> MYDFTNC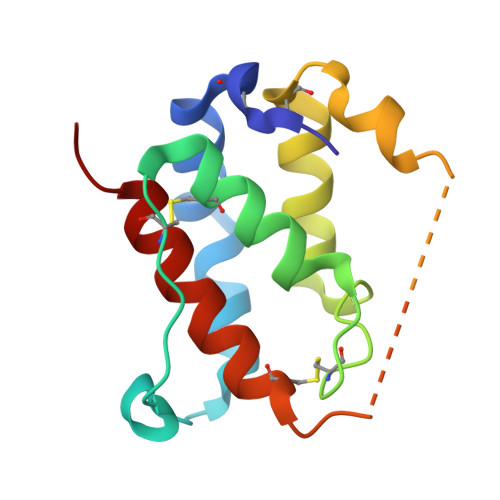DFEKIKAAYLSTISKDLITYMSGTKSTEFNNTVSCSNRPHCLTEIQSLTFNPTAGCASLAKEMFAMKTKAALAIWCPGYSETQINATQAMKKRRKRKVTTNKCLEQVSQLQGLWRRFNRPL6-ethenyl-N,N-dimethyl-2-(methylsulfonyl)pyrimidin-4-amine | C9 H13 N3 O2 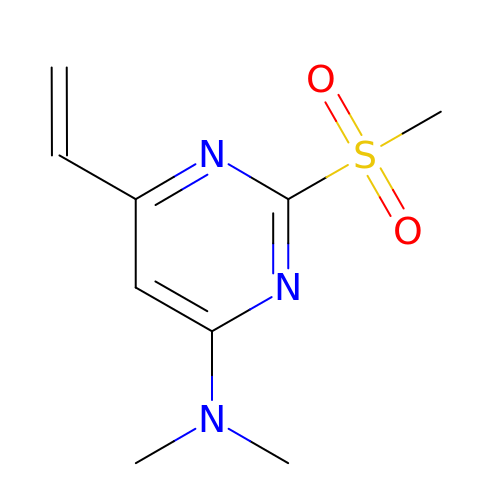S | LWXYVFFCCMAZFC-UHFFFAOYSA-N> AHHHHHHGSSTRGDLIRILGEIEEKMNE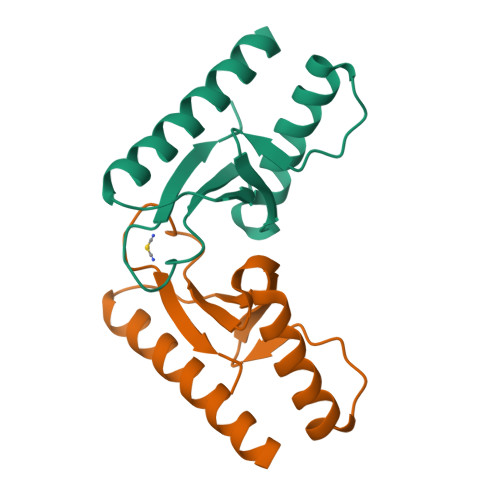LKMDGFNPDIILFGREAYNFLSNLLKKEMEEEGPFTHVSNIKIEILEELGGDAVVIDSKVLGLVPGAAKRIKIIK The enzymatic oxidation of aniline for the synthesis of conducting PANI constitutes an environmentally friendly alternative to the chemical polymerization because it is carried out under milder conditions. Even if peroxidases and laccases have been both explored as biocatalysts for aniline polymerization, laccases offer important operational advantage over peroxidases as they do not require stepwise addition of hydrogen peroxide to catalyze the reaction. Besides, peroxidases are sensitive to inactivation by hydrogen peroxide whereas laccases only require oxygen from the air to oxidize the arylamine, releasing water as the only by-product. Laccase oxidizes aniline monomers, dimers and oligomers.

The oxidation of aniline by laccase at pH 3 is hampered because at this pH aniline is mostly protonated, in the form of anilinium cation (pKa = 4.6), and the cation (E° = 1.05 V) is much less oxidizable than neutral aniline (E° = 0.63 V). Even so, the polymerization reaction with high-redox potential laccases proceeds slowly, in several hours. To sum up, even though SDBS was the anionic surfactant producing the strongest loss of enzyme activity, it endowed the best performance as doping template for the enzymatic synthesis of green PANI. Hence, 5 mM SDBS as template was fixed for the next polymerization assay with increasing amounts of 7D5 laccase and 15mM of aniline. The maximum polymerization rate (measured by the increase of polaron signal at 800 nm) was remarkably raised (0.37 < 6.37 < 14.64 mUA/min) in direct correlation with the amount of enzyme used (0.1 < 1 < 2 U/mL), suggesting the catalytic role of the enzyme in the polymerization. In all cases, polymerization slowed down from roughly 8–12 h onwards, most probably due to the inactivation of the enzyme. On the contrary, enzymatic polymerization in the presence of SDBS as template led to a nanofiber-structured PANI. By using a first-class laccase and SDBS as template, we developed an environmentally-friendly method to produce water-soluble conductive PANI with excellent electrochemical properties in up to 75% conversion yield. Its nanofibered structure provides additional advantages like a porous structure and a large surface-to-volume ratio.

>SIGPVADLTISNGAVSPDGFSRQAILVNDVFPSPLITGNKGDRFQLNVIDNMTNHTMLKSTSIHWHGFFQHGTNWADGPAFVNQCPISTGHAFLYDFQVPDQAGTFWYHSHLSTQYCDGLRGPIVVYDPQDPHKSLYDVDDDSTVITLADWYHLAAKVGPAAPTADATLINGLGRSINTLNADLAVITVTKGKRYRFRLVSLSCDPNYTFSIDGHSLTVIEADGVNLKPQTVDSIQIFPAQRYSFVLNADQDVDNYWIRALPNSGTRNFDGGVNSAILRYEGAAPVEPTTSQTPSTQPLVESALTTLEGTAAPGNPTPGGVDLALNMAFGFAGGRFTINGASFTPPTVPVLLQILSGAQSAQDLLPSGSVYSLPANADIEISLPATSAAPGFPHPFHLHGHTFAVVRSAGSSTYNYANPVYRDVVNTGSPGDNVTIRFRTDNPGPWFLHCHIDFHLDAGFAVVMAEDTPDVAATNPVPQAWSDLCPTYDALSPDDQ[2x]>MGVFTFEDEITSTV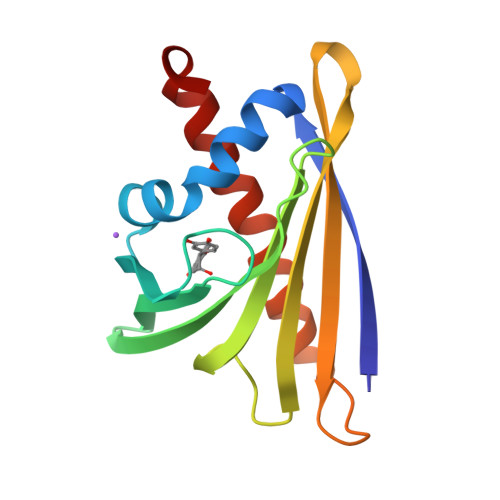PPAKLYNAMKDADSITPKIIDDVKSVEIVEGNGGPGTIKKLTIVEDGETKFILHKVESIDEANYAYNYSVVGGVALPPTAEKITFETKLVEGPNGGSIGKLTLKYHTKGDAKPDEEELKKGKAKGEGLFRAIEGYVLANPTQY[2x]> MATEFGTAVNHADLVERLVQFLTASPDLVAAGQAYEKVFDNTIPASGTAIAVRQVTLRAPGLGGTDAIYMGIQSYGDTALDYYNLRLMGGTAFNPGAIPPGGDYWTAFANY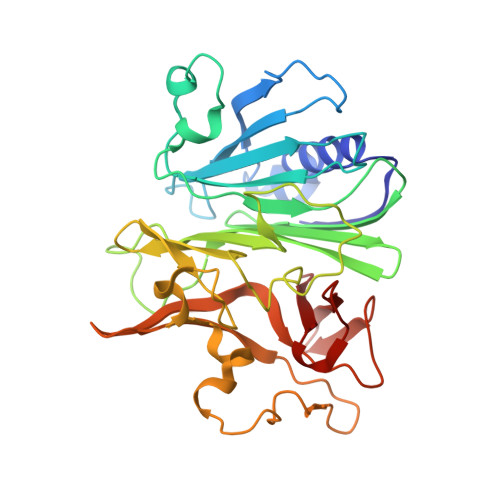SPRVQLLAWNQPMPYWFFANGRRFWIVVKVSTIYESAGAGFILPPCPPSQYPYPLAVVGSYRGDVATRWSDVSDRHRGISSPYERSCYLRDPAGRWLGFTVDGGAANESDYNNRTLLPLGCGRYAGSSDTVVKQLRDSFGKFPLKALQFVTRETEGRRYLGDFDGAFYVPTLNSGAEDVIVEDGVDHVVFQTAWRSGNPWLYAIRKD> DDAAIQQTLAKMGIKSSDIQPAPVAGMKTVLT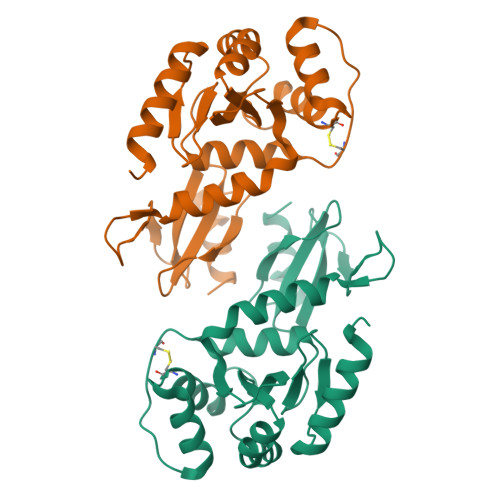NSGVLYITDDGKHIIQGPMYDVSGTAPVNVTNKMLLKQLNALEKEMIVYKAPQEKHVITVFTDITCGYCHKLHEQMADYNALGITVRYLAFPRQGLDSDAEKEMKAIWCAKDKNKAFDDVMAGKSVAPASCDVDIADHYALGVQLGVSGTPAVVLSNGTLVPGYQPPKEMKEFLDEHQKMTSGK> GEIEKRQEENRKDREKAAAKFREYFPNFVGEPKSKDILKLRLYEQQHGKCLYSGKEINLGRLNEKGYVEIDHALPFSRTWDDSFNNKVLVLGSENQNKGNQTPYEYFNG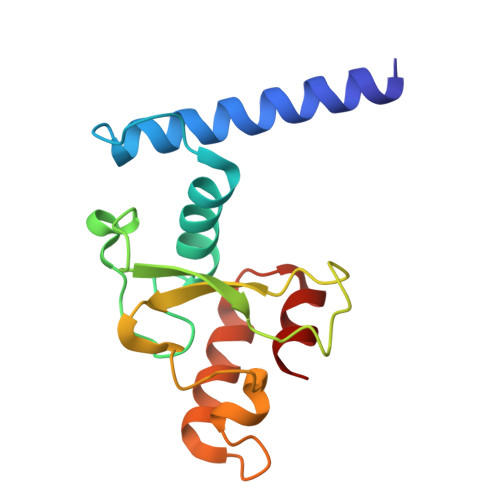KDNSREWQEFKARVETSRFPRSKKQRILLQ>TFGTFQDAYLSQLRDIYHSPEFRNAPRGQASRERIGAGFRLLDPVQRHISVPARR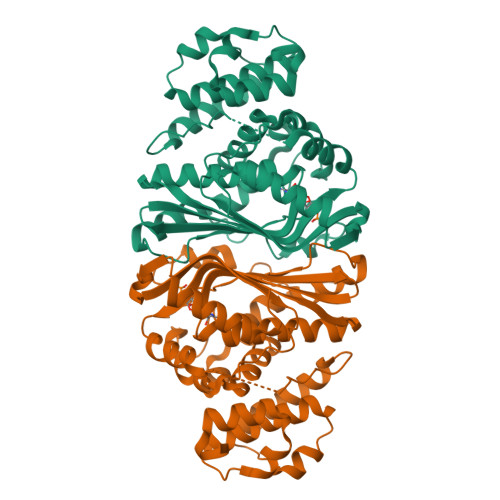ANVVFNFAEALWYLSGSDRLDFIQYYAPGIAAYSADGRTLRGTAYGPRIFRHPAGGVNQWENVVKTLTDDPDSKRAVIQIFDPRELAVADNIDVACTLALQFLIRDGLLCGIGYMRANDAFRGAVSDVFSFTFLQEFTARYLGLGIGTYHHVVGSVHIYDSDARWAERVLDAATPDGGPRPGFPAMPDGDNWPHVRRVLEWEERLRTNAARLSADALDALDLPAYWKHVVALFEAHRQVRHEDTPDRALLAALPEVYRQSLAVKWPGHFG[2x]SPS catalyzes sucrose-6-phosphate (S6P) synthesis by using UDP-glucose and fructose-6-phosphate. All SPSs identified so far belong to the GT-B type glucosyltransferase family and contain two Rossmann-type folds. The N-terminal fold is called the A-domain and the C-terminal fold is called the B-domain. Thermosynechococcus elongatus SPS is a kind of sucrose-phosphate synthase (EC 2.4.1.14).

In the present study, we solved the co-crystal structure of Thermosynechococcus elongatus SPS (TeSPS) (Uniprot code: tll1590) with S6P and UDP. Although crystallization of TeSPS alone was unsuccessful, addition of UDP did induce crystal growth, indicating that this ligand stabilized the protein for crystallization. Therefore, we decided to soak the TeSPS:UDP co-crystals with S6P in an attempt to stabilze the structure further and increase resolution. In doing so, we were able to obtain a dataset at 3 Å resolution. The crystal structure of TeSPS (residues 27–426) showed that it is a GT-B type glycotransferase as a monomer. Overall, our resolved structure showed that TeSPS has 16 α helices and 14 β sheets, with UDP and S6P being bound at the interface of A- and B-domains. The N-terminus (residues 27–220) and the α6 helix (residues 406–426) formed the A-domain, and the C-terminus (residues 221–405) formed the B-domain, with two loops (connecting α6 and α6’ and α7’ and β8, respectively) linking these two domains. In our structure, TeSPS is in the closed conformational state. In particular, UDP and S6P stabilize conformations of the loops in the catalytic center in which the uracil moiety of UDP is inserted into a cavity formed by loops 1, 3, 4, and 5. Hydrophobic residue Leu335 that is proximal to two phosphate groups from UDP is forced to reorient, and the terminal phosphate (P1) of UDP is stabilized by interactions with basic amino acids, including Arg249 and Arg253.

>GSHMQALSTRTAKNTLPRAFAMPQPQVPARQPIALISVHGDPAADVGHESAGGQNIYVRQLGEALAAAGWHVDMFTRKTDPNDPDVIEHSPHCRTIRLQAGPLTYIPREKLFETLPKFVEAFKAYHAKYGYPLIHTNYWLSGWVGWQLRQQFNFQWLHTYHSLGVVKYQVASEQAQRDETRLMVEKAILENADCVIVTSPQEEAYLRRWVSKAGQTRLIPCGTNLKLFYPVADARAQLNLPADEPIVLYVGRFDRRKGIETLVAAMAQIPQGQLLLVGGSDPQRSDGAERRRIEGLVQEYNLGDRVTFVGQIDHEYLAVYYSAANVCVVPSYYEPFGLVAIEAMACGTPVIASAVGGLQFTVIPEETGLLVPPQDANALANAIQRILADPAWARTLGKNGRERVQALFNWEAIALQMGQLYRQLFAASLMGNSPRLEMVKNTASLAAVTKAALAS[12x]> MTYSQTYAAWKNDPEGFWMEAAQAIDWVTPPGAALNSDNAPLYEWFTDAEVNTCFNAVDRHVQAGNGDRVAIIHDSPVTHTKQEITYAELQERVSLLAGALRAKGIEKGDRVLIYMPMVPQALEAMLACARLGAIHSVVFGGFAANELAVRIDDATPKAIIAASCGIEPGRVVHYKPLLDGAIDLATHKPDFCLIFQREQEVAHLEPGRDFDWHEAQYGVDPAECVPVAGNHPAYILYTSGTTGQPKGVLRPTAGHLVALNWTMKNIYNVD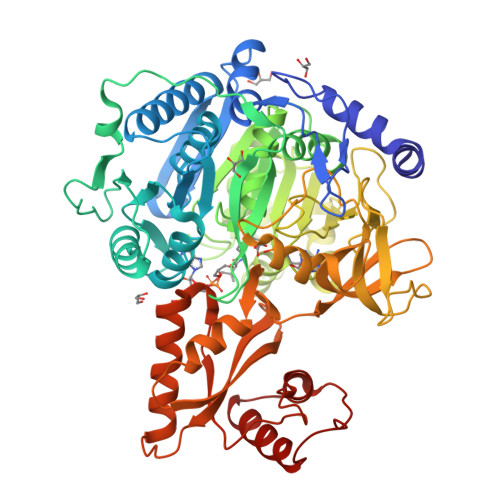PGDVFWAASDVGWVVGHSYICYAPLIHGNTTIVFEGKPVGTPDAGTFWRVISEHKVKSFFTAPTALRAVKREDPNGEFIGKYDLSHLKTVYLAGERADPDTIQWTMDKLGVPVIDHWWQTETGWAIAANPMGIEHLPVKIGSPSVAMPGYDVQVLDEGGHPVAPGTLGAIAVKLPLAPGTLPNLWQAEERFVKSYLTTFPGYYETGDAGYIDEDGYLYIMARTDDVINVAGHRLSTGAMEEVLASHPDVAECAVIGVSDTLKGQMPLGFLCLSAGVNRPHDEIAKECVKLVREKIGPVAAFKLACVVDRLPKTRSGKILRGTMVNIADGTPWKMPATIDDPAILDEITEALGKLGYPAS> MEVVSLPRLGEPAPAFEAQTTFGPVKFPDDFKGQWVVLFSHPADFTPVCTTEFVAFAKNYEEFKKRNVQLIGLSVDSNFSHIAWVMNIKEKFGIEIPFPIIADHNMEVAKKYGMIHPAQSTTFTVRALFVIDDKGILRAMIYYPLTTGRNIREV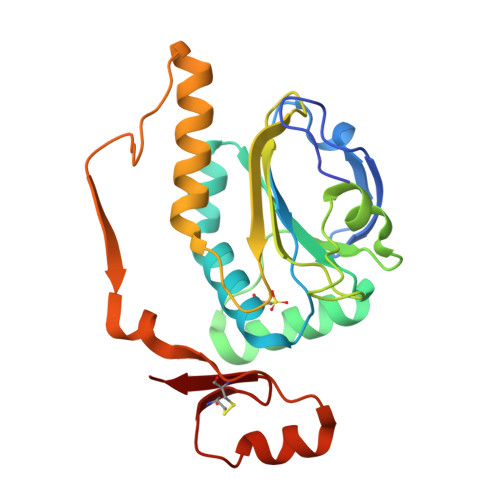IRLVDALQTADREGVATPADWVPEPQTWEFTEENTKVIVPPPTTYEDAVKRLQEGYECADWYICKKKV> GSHMYEYPVFSHVQAGMFSPELRTFTKGDAERWVSTTKKASDSAFWLEVEGNSMTTPTGSKTSFPDGMLILVDPEQAVEPGDFCIARLGGDEFTFKKLIRDSGQVFLQPLNPQ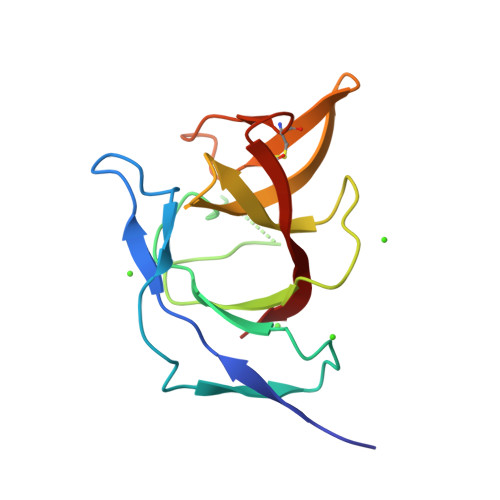YPMIPCNESCSVVGKVIASQ> SHMASMKKKGSVVIVGRINLSGDTAYAQQTRGEEGCQETSQTGRDKNQVEGEVQIVST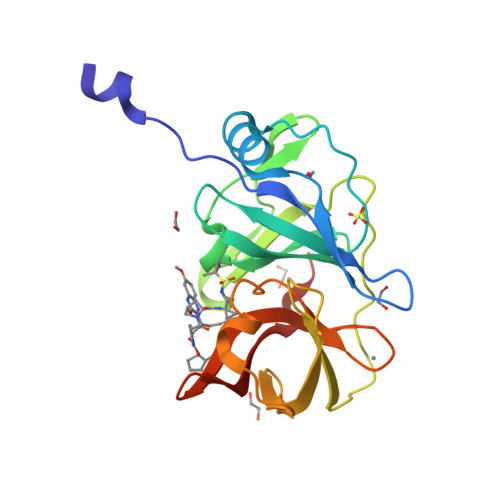ATQTFLATSINGVLWTVYHGAGTRTIASPKGPVTQMYTNVDKDLVGWQAPQGSRSLTPCTCGSSDLYLVTRHADVIPVRRRGDSRGSLLSPRPISYLKGSSGGPLLCPAGHAVGIFRAAVSTRGVAKAVAFIPVESLETTM> SMFNSEIKEKYLDTLSEGMVMQMRPIFAKAEITETLYNKDIYDFTSMQILELIRSFDQTTIGSVRRTLALLSLYIDWAISYKLSKGLTNLARTISEEELYECLGDKKLYITYSELEEMENQLVNYQSKAVLRLLFEGVSGLAHSELLSLTKKQVEDAMLNGNVLTLYDSKHGERKLKVSSECLVIALNAAQETKYKLKNGKAKGQTKEVFLVENDYVVKTKRTSNKGDGQASKFVITNLITDISEFFKINFLTPNTIVRSGHLYRAYQLYKEKGVIDNSVRYQIIDDFNLRVKSKYRAVYSMQDYINEEEVNKY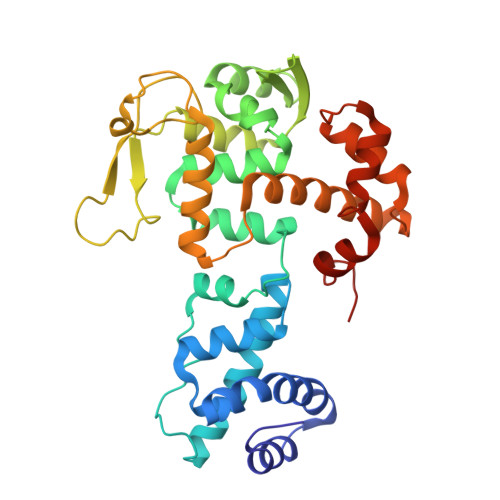YAEELGLKETTI The second principal receptor for IgE, CD23, is a type II transmembrane glycoprotein with a C-type lectin-like domain (CTLD)4 (3, 4). In its membrane-bound form, CD23 consists of three CTLD “heads” connected to the membrane via a trimeric α-helical coiled-coil “stalk”. The interaction between CD23 and IgE is critical in the regulation of IgE synthesis, which can be up- or down-regulated depending on the oligomerization state of CD23 (2, 9, 10). We have determined the crystal structures of the human lectin-like head domain of CD23 in its Ca2+-free and Ca2+-bound forms, as well as the crystal structure of the Ca2+-bound head domain of CD23 in complex with a subfragment of IgE-Fc consisting of the dimer of Cϵ3 and Cϵ4 domains (Fcϵ3-4).

To resolve the controversy, the crystal structure of Ca2+-bound wild-type human derCD23 was solved. Unlike MBL and DC-SIGN that bind two and three Ca2+ ions, respectively, Ca2+-soaked human derCD23 crystals reveal that a single Ca2+ ion binds at the principal binding site in all four molecules of the asymmetric unit. The electron density for the Ca2+-coordinating ligands (Glu-249, Thr-251, Asp-270, and three water molecules) and the Ca2+ ion itself is well defined in three of the derCD23 molecules; electron density for the three water molecules and Thr-251 in the fourth molecule is unclear. In the wild-type Ca2+-bound derCD23 crystal structure presented here, three residues (Glu-249, Thr-251, and Asp-270) provide four oxygen atoms, and three water molecules provide a further three for the binding of Ca2+. The coordination geometry is pentagonal bipyramidal formed by the seven ligands. Surprisingly, in contrast to Wurzburg et al., we found that the highly conserved Asn-269 residue is not directly involved in the binding of Ca2+; the nitrogen atom of the carboxamide group was found to form a hydrogen bond with a water molecule that acts as a Ca2+ ligand. Additionally, we found that three water molecules, not two as previously suggested, directly ligate Ca2+. In the Ca2+-bound structure, Pro-250 adopts a cis configuration in all four copies, and the distance between Thr-251 (Oγ1) and Glu-249 (Oϵ1) is 3.7 Å. In the presence of Ca2+, Pro-250 is effectively locked into the cis configuration. The structure of Ca2+-bound derCD23 reported here shows a single ion bound at the principal calcium site, liganded by Glu-249, Thr-251, Asp-270, and three water molecules; the KD is 1.5 mm.

>[4x]SGFVCNTCPEKWINFQRKCYYFGKGTKQWVHARYACDDMEGQLVSIHSPEEQDFLTKHASHTGSWIGLRNLDLKGEFIWVDGSHVDYSNWAPGEPTSRSQGEDCVMMRGSGRWNDAFCDRKLGAWVCDRLATCTPPASEGSAE>[4x]GEIRPTIGQQMETGDQRFGDLVFRQLAPNVWQHTSYLDMPGFGAVA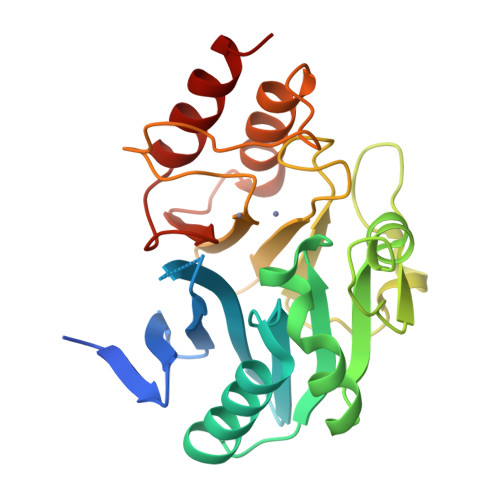SNGLIVRDGGRVLVVDTAWTDDQTAQILNWIKQEINLPVALAVVTHAHQNKMGGMDALHAAGIATYANALSNQLAPQEGMVAAQHSLTFAANGWVEPATAPNFGPLKVFYPGPGHTSDNITVGIDGTDIAFGGCLIKDSKAKSLGNLGDADTEHYAASARAFGAAFPKASMIVMSHSAPDSRAAITHTARMADKLR>MAVKVIVTDMDGTFLNDAKTYNQPRFMA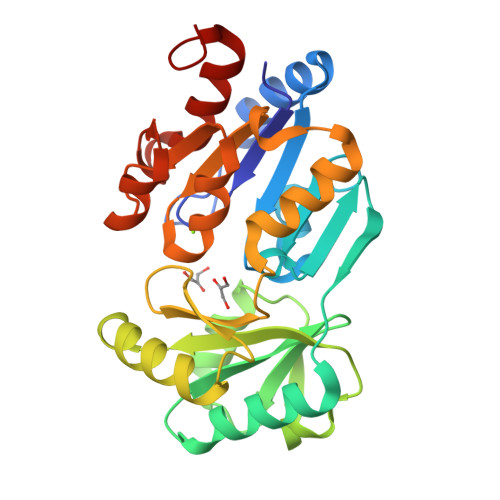QYQELKKRGIKFVVASGNQYYQLISFFPELKDEISFVAENGALVYEHGKQLFHGELTRHESRIVIGELLKDKQLNFVACGLQSAYVSENAPEAFVALMAKHYHRLKPVKDYQEIDDVLFKFSLNLPDEQIPLVIDKLHVALDGIMKPVTSGFGFIDLIIPGLHKANGISRLLKRWDLSPQNVVAIGDSGNDAEMLKMARYSFAMGNAAENIKQIARYATDDNNHEGALNVIQAVLDNTYPFNS[4x]AppA, the Escherichia coli periplasmic phytase of clade 2 of the histidine phosphatase (HP2) family, has been well-characterized and successfully engineered for use as an animal feed supplement. The E. Coli periplasmic phytase, AppA, is a 1D-6-phytase (EC 3.1.3.2) and initial hydrolysis preferentially liberates the phosphate at the 1D-6-position on the inositol ring. HP2Ps catalyse the hydrolysis of phytate via an obligatory phosphohistidine intermediate. The catalytic proton donor is found in a second, short, conserved motif with sequence HD positioned such that the aspartic acid residue functions as the consensus proton donor in the catalytic mechanism.

As phytate is rapidly hydrolysed by wild-type AppA, our efforts to capture crystallographic snapshots of its complex with the substrate by soaking crystals with InsP6 were unsuccessful. This was the case even at pHs where the enzyme retains minimal activity in solution, yielding only the structure of the orthophosphate (product)-bound complex. Utilizing this structure as a proxy for the enzyme in the covalent intermediate state, the structure of the wild-type enzyme with InsS6 as representative of its complex with phytate, and the structure of the complex of the enzyme with orthophosphate as representative of the complex with the second stage product, we can now build on previous descriptions of conformational changes occurring during catalysis to describe snapshots during the complete structural catalytic cycle of the enzyme. Notably, the involvement of R20 in stabilizing the phosphohistidine intermediate and its interactions with bound orthophosphate in the product complex explain why loop opening does not occur until after loss of the second stage product. We also observed a conformational change in the sidechain of E219 on binding of the pseudosubstrate inhibitor and found this water site conserved in the structure of the complex with orthophosphate.

> GPQSEPELKLESVVIVSRHGVRAPTKATQLMQDVTPDAWPTWPVKLGWLTPRGGELIAYLGHYQRQRLVADGLLAKKGCPQSGQVAIIADVDERTRKTGEAFAAGLAPDCAITVHTQADTSSPDPLFNPLKTGVCQLDNANVTDAILSRAGGSIADFTGHRQTAFRELERVLNFPQSNLCLKREKQDESCSLTQALPSELKVSADNVSLTGAVSLASMLTEIFLLQQAQGMPEPGWGRITDSHQWNTLLSLHNAQFYLLQRTPEVARSRATPLLDLIKTALTPHPPQKQAYGVTLPTSVLFIAGHDTNLANLGGALELNWTLPGQPDNTPPGGELVFERWRRLSDNSQWIQVSLVFQTLQQMRDKTPLSLNTPPGEVKLTLAGCEERNAQGMCSLAGFTQIVNEARIPACSL>MAELPTTETPGDATLCSGRFTISTLLSSDEPSPPAAYDSSHPSHLTHSSTFCMRTFGYNTIDVVPTYEHYANSTQPGEPRKVRPTLADLHSFLKEGRHLHALAFDSRPSHEMTDGLVEGEAGTSSEKNPEEPVRFGWVKGVMIRCMLNIWGVILYLRLPWITAQAGIVLTWIIILLSVTVTSITGLSISAISTNGKVKSGGTYFLISRSLGPELGGSIGLIFAFANAVGVAMHTVGFAETVRDLLQEYGAPIVDPINDIRIIAVVSVTVLLAISLAGMEWESKAQVLFFLVIMVSFANYLVGTLIPPSEDKASKGFFSYRADIFVQNLVPDWRGPDGTFFGMFSIFFPSATGILAGANISGDLKDPAIAIPKGTLMAIFWTTISYLAISATIGSCVVRDASGVLNDTVTPGWGACEGLACSYGWNFTECTQQHSCHYGLINYYQTMSMVSGFAPLITAGIFGATLSSALACLVSAAKVFQCLCEDQLYPLIGFFGKGYGKNKEPVRGYLLAYAIAVAFIIIAELNTIAPIISNFFLCSYALINFSCFHASITNSPGWRPS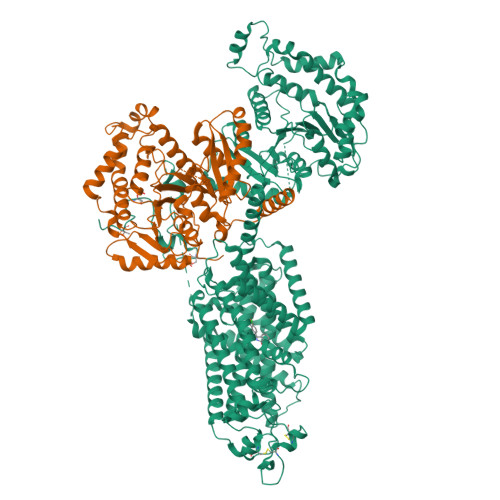FQYYNKWAALFGAIISVVIMFLLTWWAALIAIGVVLFLLLYVIYKKPEVNWGSSVQAGSYNLALSYSVGLNEVEDHIKNYRPQCLVLTGPPNFRPALVDFVGTFTRNLSLMICGHVLIGPHKQRMPELQLIANGHTKWLNKRKIKAFYSDVIAEDLRRGVQILMQAAGLGRMKPNILVVGFKKNWQSAHPATVEDYIGILHDAFDFNYGVCVMRMREGLNVSKMMQAHINPVFDPAEDGKEASARVDPKALVKEEQATTIFQSEQGKKTIDIYWLFDDGGLTLLIPYLLGRKRRWSKCKIRVFVGGQINRMDQERKAIISLLSKFRLGFHEVHILPDINQNPRAEHTKRFEDMIAPFRLNDGFKDEATVNEMRRDCPWKISDEEITKNRVKSLRQVRLNEIVLDYSRDAALIVITLPIGRKGKCPSSLYMAWLETLSQDLRPPVILIRGNQENVLTFYCQ[2x]>MAAFKPNSINYILGLDIGIASVGWAMVEIDEEENPIRLIDLGVRVFERAEVPKTGDSLAMARRLARSVRRLTRRRAHRLLRTRRLLKREGVLQAANFDENGLIKSLPNTPWQLRAAALDRKLTPLEWSAVLLHLIKHRGYLSQRKNEGETADKELGALLKGVAGNAHALQTGDFRTPAELALNKFEKESGHIRNQRSDYSHTFSRKDLQAELILLFEKQKEFGNPHVSGGLKEGIETLLMTQRPALSGDAVQKMLGHCTFEPAEPKAAKNTYTAERFIWLTKLNNLRILEQGSERPLTDTERATLMDEPYRKSKLTYAQARKLLGLEDTAFFKGLRYGKDNAEASTLMEMKAYHAISRALEKEGLKDKKSPLNLSPELQDEIGTAFSLFKTDEDITGRLKDRIQPEILEALLKHISFDKFVQISLKALRRIVPLMEQGKRYDEACAEIYGDHYGKKNTEEKIYLPPIPADEIRNPVVLRALSQARKVINGVVRRYGSPARIHIETAREVGKSFKDRKEIEKRQEENRKDREKAAAKFREYFPNFVGEPKSKDILKLRLYEQQHGKCLYSGKEINLGRLNEKGYVEIDHALPFSRTWDDSFNNKVLVLGSENQNKGNQTPYEYFNGKDNSREWQEFKARVETSRFPRSKKQRILLQKFDEDGFKERNLNDTRYVNRFLCQFVADRMRLTGKGKKRVFASNGQITNLLRGFWGLRKVRAENDRHHALDAVVVACSTVAMQQKITRFVRYKEMNAFDGKTIDKETGEVLHQKTHFPQPWEFFAQEVMIRVFGKPDGKPEFEEADTLEKLRTLLAEKLSSRPEAVHEYVTPLFVSRAPNRKMSGQGHMETVKSAKRLDEGVSVLRVPLTQLKLKDLEKMVNREREPKLYEALKARLEAHKDDPAKAFAEPFYKYDKAGNRTQQVKAVRVEQVQKTGVWVRNHNGIADNATMVRVDVFEKGDKYYLVPIYSWQVAKGILPDRAVVQGKDEEDWQLIDDSFNFKFSLHPNDLVEVITKKARMFGYFASCHRGTGNINIRIHDLDHKIGKNGILEGIGVKTALSFQK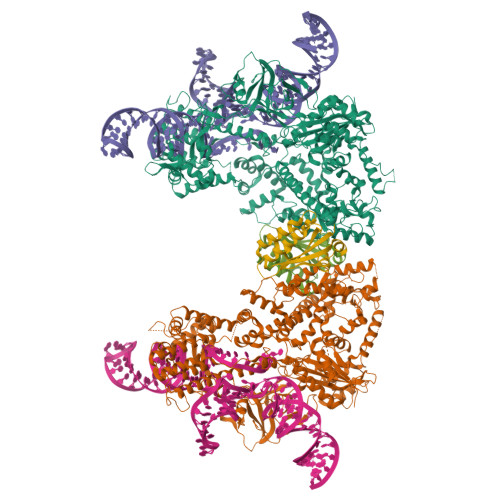YQIDELGKEIRPCRLKKRPPVRSEHHHHHHHH[2x];>[2x]SMFKRAIIFTSFNGFEKVSRTEKRRLAKIINARVSIIDEYLRAKDTNASLDGQYRAFLFNDESPAMTEFLAKLKAFAESCTGISIDAWEIEESEYVRLPVERRDFLAAANGKEIFKI> ATKKAV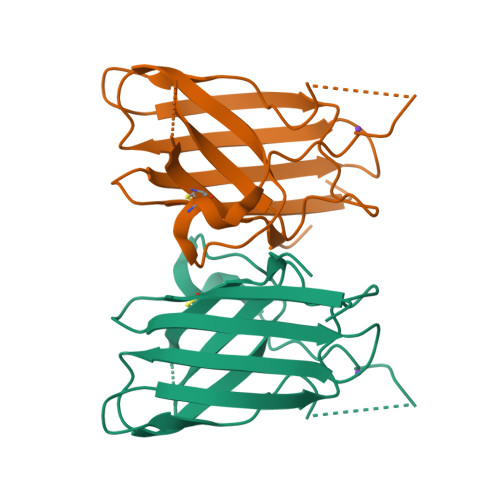AVLKGNSNVEGVVTLSQDDDGPTTVNVRITGLAPGLHGFHLHEYGDTTNGCMSTGAHFNPNKLTHGAPGDEIRHAGDLGNIVANADGVAEVTLVDNQIPLTGPNSVVGRALVVHELEDDLGKGGHELSLTTGNAGGRLACGVVGLTPI> NPKSLTRGPRDKPTPLEELLPHAIEFINQYYGSFKEAKIEEHLARLEAVTKEIETTGTYQLTLDELIFATKMAWRNAPRCIGRIQWSNLQVFDARNCSTAQEMFQHICRHILYATNNGNIRSAITVFPQRSDGKHDFRLWNSQLIRYAGYQMPDGTIRGDAATLEFTQLCIDLGWKPRYGRFD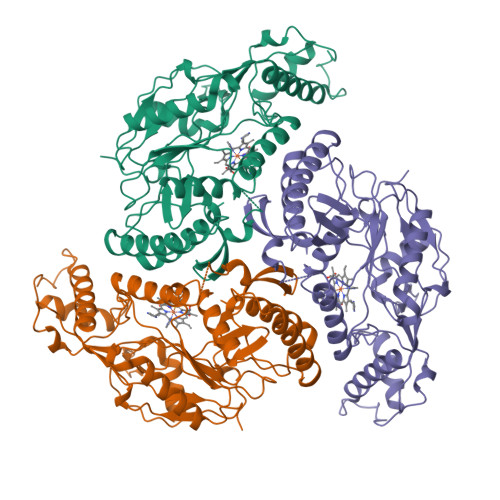VLPLVLQADGQDPEVFEIPPDLVLEVTMEHPKYEWFQELGLKWYALPAVANMLLEVGGLEFPACPFNGWYMGTEIGVRDFCDTQRYNILEEVGRRMGLETHTLASLWKDRAVTEINVAVLHSFQKQNVTIMDHHTASESFMKHMQNEYRARGGCPADWIWLVPPVSGSITPVFHQEMLNYVLSPFYYYQIEPWKTHIWQNEHHHH;> MEKKITGYTTVDISQWHRKEHFEAFQSVAQCTYNQTVQLDITAFLKTVKKNKHKFYPAFIHILARLMNAHPEFRMAMKDGELVIWDSVHPCYTVFHEQTETFSSLWSEYHDDFRQFLHIYSQDVACYGENLAYFPKGFIENMFFVSANPWVSFTSFDLNVANMDNFFAPVFTMGKYYTQGDKVLMPLAIQVHHAVCDGFHVGRMLNELQQYCDEWQGGA methyl 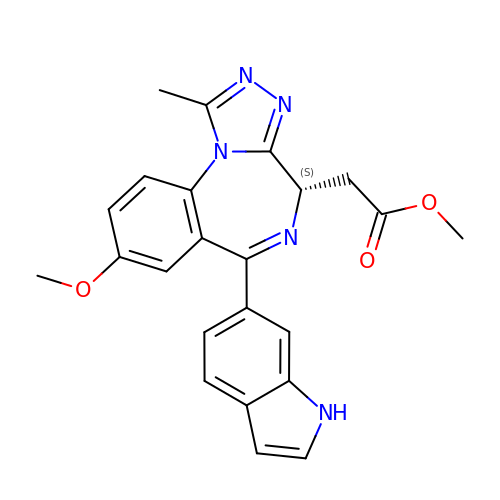[(4S,6P,10aM)-6-(1H-indol-6-yl)-8-methoxy-1-methyl-4H-[1,2,4]triazolo[4,3-a][1,4]benzodiazepin-4-yl]acetate | C23 H21 N5 O3 | LKJBIUFJSLTBCA-IBGZPJMESA-N> MNLPTAQEVQGLMARYIELVDVGDIEAIVQMYADDATVEDPFGQPPIHGREQIAA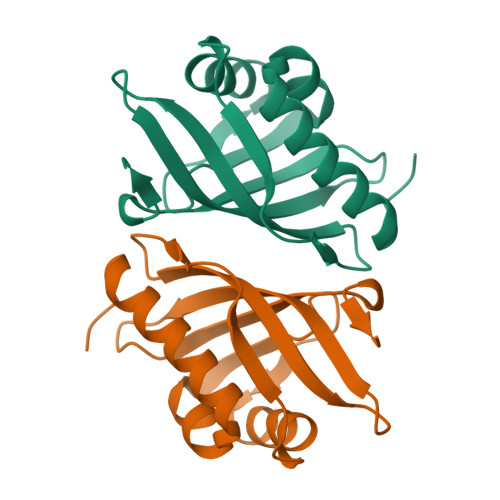FYRQGLGGGKVRACLTGPVRASHNGCGAMPFRVEMVWNGQPCALDVIDVMRFDEHGRIQTAQAYWSEVNLSVREPQ> MNAYYIQDRLEAQSWARHYQQLAREEKEAELADDMEKGIPQHLFESLCIDHLQRHGASKKSITRAFDDDVEFQE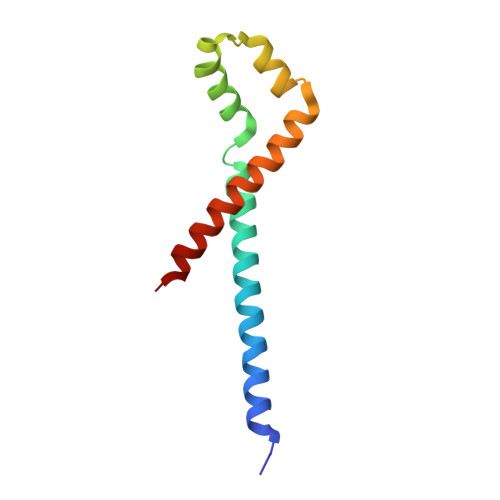RMAEHIRYMVETIAHHQVDIDSEV Here, we presented structural and phylogenetic analyses of two meropenem-sensitive Mtb penicillin-binding proteins, Rv2911 and Rv3330. A search of the Mtb genome for Peptidase_S11 Pfam family proteins (PF00768) yielded two hits: Rv2911 and Rv3330. The active sites of both proteins contain the three typical penicillin-binding protein motifs: SXXK, SXN, and KTG. The structures showed similar overall folds containing two subdomains.

Rv3330 was bound to meropenem, a beta-lactam antibiotic that was added prior to crystallization. The Rv2911opt-PMSF structure was determined at 2.0 Å resolution using multiwavelength anomalous dispersion of Se-labeled enzyme. This structure was used as the search model to determine the Rv3330-meropenem structure, also at 2.0 Å resolution. In contrast, upon binding to Rv3330, the meropenem molecule assumed a single conformation, as demonstrated by a well-defined electron density envelope extending away from the active site. This unique conformation is stabilized by several key interactions. First, the alanine-like moiety within meropenem is hydrogen bonded to Thr283 through the carboxyl and to Ser176 through both the carboxyl and amide groups. This interaction mimics the contacts made by the D-alanine leaving group of the natural pentapeptide substrate. Third, the π-system of the distal carbamoyl moiety participates in a stacking interaction with the phenyl ring of Tyr284. Finally, the oxygen of the carbamoyl group is hydrogen bonded to Asn291 and Arg313, two residues outside of the canonical active site motifs that are nonetheless universally conserved among mycobacterial orthologs of Rv3330. In contrast, the distal end of this inhibitor, which is variable in carbapenems, points away from the stem peptide-binding site. In the Rv3330 crystals, Cys77 residues from adjacent molecules formed a disulfide across a two-fold axis.

> GHMPYKVSTPPAVDSSEVPAAGEPPLPLVVPPTPVGGNALGGCGIITAPGSAPAPGDVSAEAWLVADLDSGAVIAARDPHGRHRPASVIKVLVAMASINTLTLNKSVAGTADDAAVEGTKVGVNTGGTYTVNQLLHGLLMHSGNDAAYALARQLGGMPAALEKINLLAAKLGGRDTRVATPSGLDGPGMSTSAYDIGLFYRYAWQNPVFADIVATRTFDFPGHGDHPGYELENDNQLLYNYPGALGGKTGYTDDAGQTFVGAANRDGRRLMTVLLHGTRQPIPPWEQAAHLLDYGFNTPAGTQIGTLIEPDPSLMSTDRNPADRQRVDPQAAAR>[2x]GPDAETTTHPEAFQESLKHLLPDLSDYSEITIHLLHQLVLACGDVSLVNAVRLSQGAIASARDALKAGCPVVTDVPVVA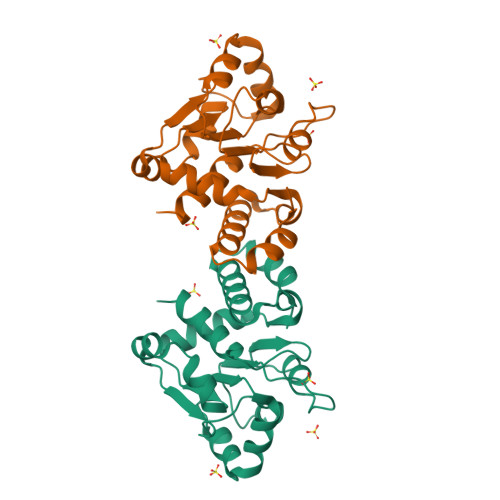AALDQTRLAHLGCTVKTLIDDPHITTAREAEQAFWHHDHWQQRLQQIPQGSVLAIGYAPSVLLTACKLIEQQHIQPALVIGMPIGFSHAPAAKRRLMTSPIPHITIQGSLGGGLLAAVALNALVETLIEKPDSHSYLTS> GHMSTPRPSLTLTLLQAREAAMSFFRPSLNQHGLTEQQWRVIRILRQQGEMESYQLAN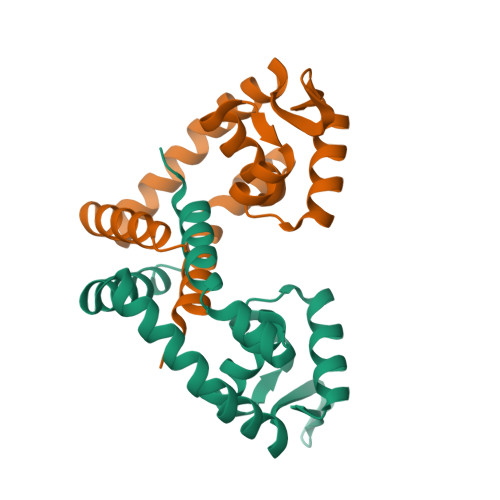QACILRPSMTGVLARLERDGIVRRWKAPKDQRRVYVNLTEKGQQCFVSMSGDMEKNYQRIQERFGEEKLAQLLELLNELKKIKP>[3x]MATNFFIQPITEEAEAYYPPSVITNKRKDLGVDVYCCSDLVLQPGLNIVRLHIKVACEHMGKKCGFKIMARSSMCTHERLLILANGIGLIDPGYVGELMLKIINLGDTPVQI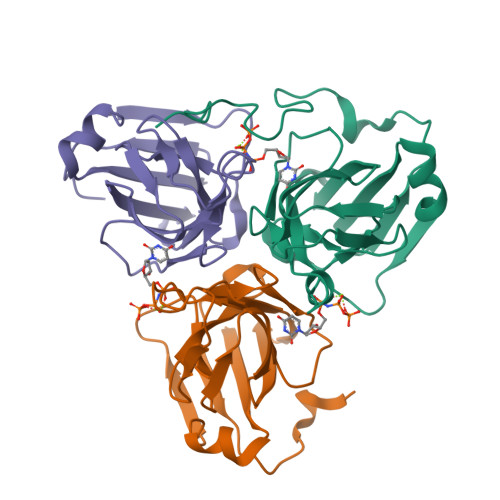WAKECLVQLVAQGDHVPDHINILKRNQIFPLFAPTPRGEGRFGSTGEAGIMRT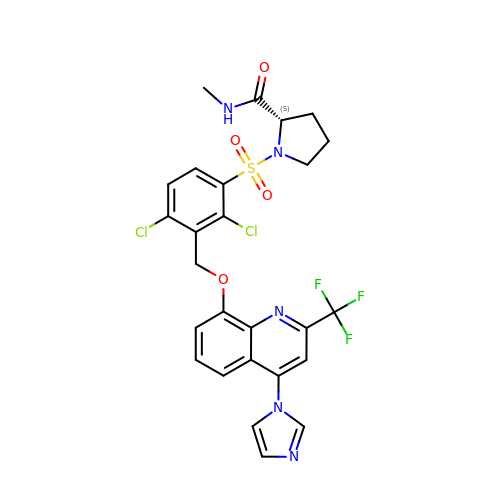(2~{S})-1-[2,4-bis(chloranyl)-3-[[4-imidazol-1-yl-2-(trifluoromethyl)quinolin-8-yl]oxymethyl]phenyl]sulfonyl-~{N}-methyl-pyrrolidine-2-carboxamide | C26 H22 Cl2 F3 N5 O4 S | YPZVBDHGFDAMKP-SFHVURJKSA-N>VPGPEYKVAILTVSDTVSAGAGPDRSGPRAVSVVDSSSEKLGGAKVVATAVVPDEVERIKDILQKWSDVDEMDLILTLGGTGFTPRDVTPEATKKV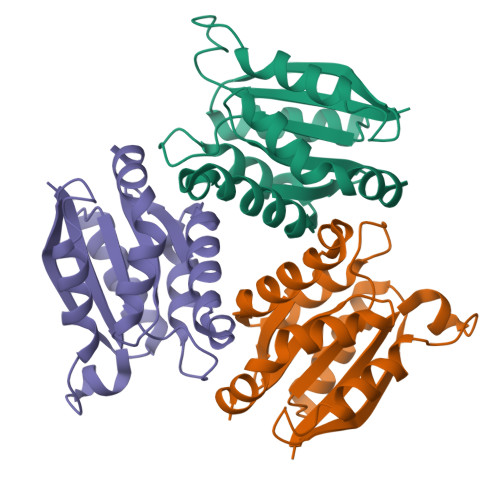IERETPGLLFVMMQEALKITPFAMLSRSAAGIRGSTLIINMPGNPNAVAECMEALLPALKHALKQIKGDKR[8x]> GSDYEFLKSWTVEDLQKRLLALDPMMEQEIEEIRQKYQSKRQPILDAIEAK;> GSEVEWDAFSIPELQNFLTILEKEEQDKIQQVQKKYDKFRQKLEEALRESQGKPG

Recent research into cellular homeostasis has shown that the Hippo signalling pathway, which is mediated by mammalian sterile 20-like kinase (MST, the human orthologue of Hippo), controls organ size in animals and regulates cell proliferation and cell death. The MST-mediated apoptosis pathway is controlled by its interaction with RASSF family proteins and the WW45 protein. Interestingly, all three classes of tumour suppressors, MST, RASSF and WW45, interact through their SARAH (SAV/RASSF/HPO) domains. We also elucidated the MST2 homodimeric structure and performed structural and biophysical comparisons of the homodimeric and heterodimeric interactions.

The crystal structure of the SARAH complex, consisting of the MST1 (residues 432–480) and RASSF5 (residues 366–418) SARAH domains, was determined by SAD from a single SeMet-derivatized crystal at the Se K edge. The MST1–RASSF5 SARAH heterodimer is characterized by head-to-tail interaction of the two protomers, forming an antiparallel helix dimer between the elongated α-helix of MST1 SARAH and the h2 helix of RASSF5 SARAH. While the SARAH domain of RASSF5 consists of two helices (h1, residues Glu66–Ser373; h2, residues Ile374–Glu412), that of MST1 has only one helix which corresponds to the h2 helix in the MST1 homodimer structure. Thus, the h2 helix in the MST1–RASSF5 heterodimer is three residues longer than that in the MST1 homodimer. These observations suggest that the h1 helix of the MST1 SARAH domain becomes unstructured and that the h2 helix extends to the N-terminus when it binds to the RASSF5 SARAH domain; this was confirmed by NMR spectroscopy in solution in the current study. The unfolding of the MST1 SARAH h1 helix in the MST1–RASSF5 heterodimeric structure may result from steric hindrance of the MST1 h1 helix by the straight RASSF5 h2 helix, which is evident in superimposed structures of the homodimers and heterodimers. Another difference in the MST1 structure between the heterodimer and the homodimer was that there was a significant distortion of the α-helix of the MST1 protomer in the MST1–RASSF5 heterodimer at proline residues Pro453 and Pro472. In addition, the side chain of Lys398 of RASSF5 was found to form a bifurcated hydrogen bond to Glu458 of MST1. Moreover, the guanidine of Arg470 of MST1 formed a bifurcated hydrogen bond to the side-chain carbonyl of Glu388 of RASSF5. Therefore, we think that the extensive hydrophobic and polar contacts in the MST1–RASSF5 complex stabilize the heterodimer structure better than they stabilize the homodimer structures. By extension of the h2 helix and unfolding of the h1 helix, the MST1 SARAH domain in the heterodimer can provide motional freedom to the MST1 catalytic domain.> MLDPNLLRNEPDAVAEKLARRGFKLDVDKLGALEERRKVLQ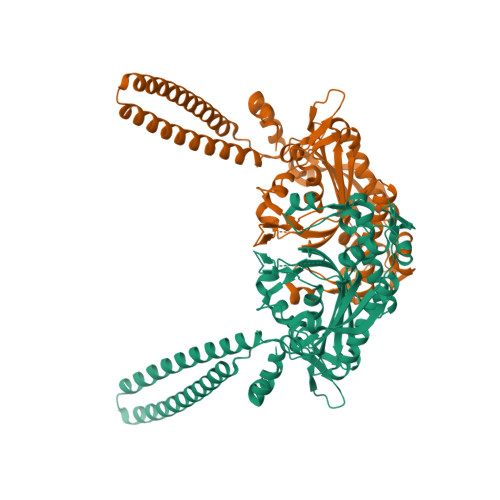VKTENLQAERNSRSKSIGQAKARGEDIEPLRLEVNKLGEELDAAKAELDALQAEIRDIALTIPNLPADEVPVGKDENDNVEVSRWGTPREFDFEVRDHVTLGEMHSGLDFAAAVKLTGSRFVVMKGQIARMHRALSQFMLDLHTEQHGYSENYVPYLVNQDTLYGTGQLPKFAGDLFHTRPLEEEADTSNYALIPTAEVPLTNLVRGEIIDEDDLPIKMTAHTPCFRSEAGSYGRDTRGLIRMHQFDKVEMVQIVRPEDSMAALEEMTGHAEKVLQLLGLPYRKIILCTGDMGFGACKTYDLEVWIPAQNTYREISSCSNVWDFQARRMQARCRSKSDKKTRLVHTLNGSGLAVGRTLVAVMENYQQADGRIEVPEVLRPYMNGLEYIG>[4x]IVGG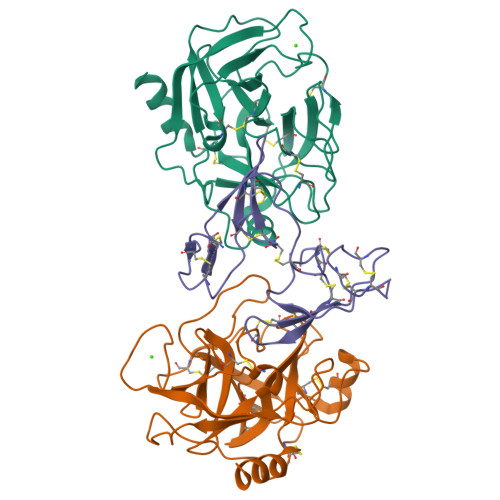YTCAANSIPYQVSLNSGSHFCGGSLINSQWVVSAAHCYKSRIQVRLGEHNIDVLEGNEQFINAAKIITHPNFNGNTLDNDIMLIKLSSPATLNSRVATVSLPRSCAAAGTECLISGWGNTKSSGSSYPSLLQCLKAPVLSDSSCKSSYPGQITGNMICVGFLEGGKDSCQGDSGGPVVCNGQLQGIVSWGYGCAQKNKPGVYTKVCNYVNWIQQTIAAN;>AGKKRPWKCCDEAVCTRSIPPICTCMDEVFECPKTCKSCGPSMGDPSRRICQDQYVGDPGPICRPWECCDKAICTRSNPPTCRCVDEVKKCAPTCKTCLPSRSRPSRRVCIDSYFGPVPPRCTPR[2x]>GPSLKSPLKPESQLDLRVQELIKLICNVQAMEEMMMEMKYNTKKAPLGKLTVAQIKAGYQSLKKIEDCIRAGQHGRALMEACNEFYTRIPHDFGLRTPPLIRTQKELSEKIQLLEALGDIEIAIKLVKTELQSPEHPLDQHYRNLHCALRPLDHESYEFKVISQYLQSTHAPTHSDYTMTLLDLFEVEKDGEKEAFREDLHNRMLLWHGSRMSNWVGILSHGLRIAPPEAPITGYMFGKGIY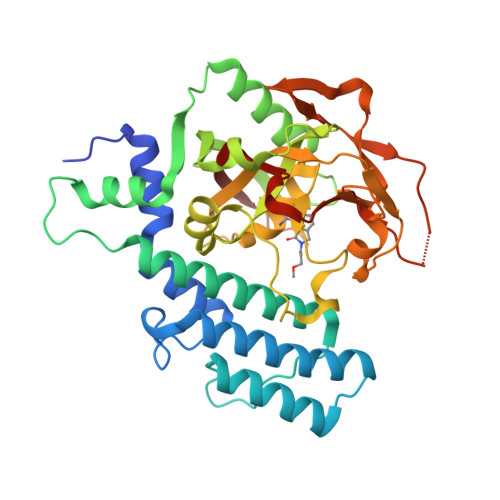FADMSSKSANYCFASRLKNTGLLLLSEVALGQCNELLEANPKAEGLLQGKHSTKGLGKMAPSSAHFVTLNGSTVPLGPASDTGILNPDGYTLNYNEYIVYNPNQVRMRYLLKVQFNFLQLW[2x]> GGCAUCGAUCCGGCGAUCACCGGGGAGCCUUCGGAAGAACGGCCGGUUAGGCCCAGUAGAACCGAACGGGUUGGCCCGUCACAGCCUCAAGUCGAGCGGCCGCGCGAAAGCGUGGCAAGCGGGGUGGCACCGCGGCGUUCGCGCGAAAGCGUGGCGUCGUCCCCGC;> GGGCCUAUAGCUCAGGCGGUUAGAG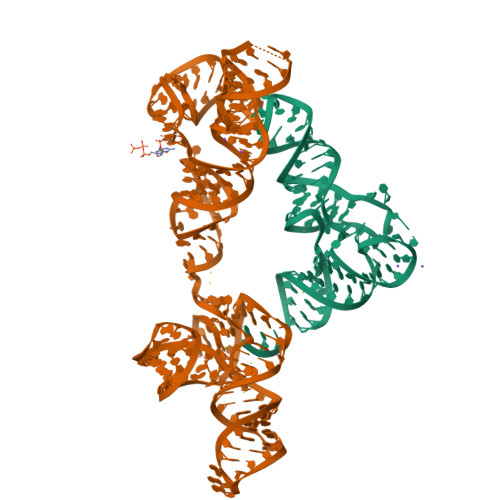CGCUUCGCUGAUAACGAAGAGGUCGGAGGUUCAAGUCCUCCUAGGCCCGCCA> EGLRVVNLLQERNMLPST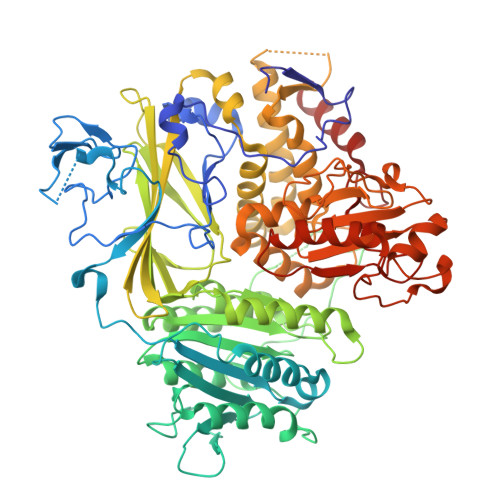PLKPPVPNLHEDIQKLNCNPELFRCTLTSIPQTQALLNKAKLPLGLLLHPFKDLVQLPVVTSSTIVRCRSCRTYINPFVSFLDQRRWKCNLCYRVNDVPEEFLYNPLTRVYGEPHRRPEVQNATIEFMAPSEYMLRPPQPPVYLFVFDVSHNAVETGYLNSVCQSLLDNLDLLPGNTRTKIGFITFDSTIHFYGLQESLSQPQMLIVSDIEDVFIPMPENLLVNLNESKELVQDLLKTLPQMFTKTLETQSALGPALQAAFKLMSPTGGRMSVFQTQLPTLGVGALKPREEPNHRSSAKDIHMTPSTDFYKKLALDCSGQQVAVDLFLLSGQYSDLASLGCISRYSAGSVYYYPSYHHQHNPVQVQKLQKELQRYLTRKIGFEAVMRIRCTKGLSIHTFHGNFFVRSTDLLSLPNVNPDAGYAVQMSVEESLTDTQLVSFQSALLYTSSKGERRIRVHTLCLPVVSTLNDVFLGADVQAISGLLANMAVDRSMTASLSDARDALVNAVIDSLSAYRSSVLSNQQPGLMVPFSLRLFPLFVLALLKQKSFQTGTNARLDERIFAMCQVKNQPLVYLMLTTHPSLYRVDNLSDEGALNISDRTIPQPPILQLSVEKLSRDGAFLMDAGSVLMLWVGKNCTQNFLSQVLGVQNYASIPQPMTDLPELDTPESARIIAFISWLREQRPFFPILYVIADESPMKANFLQNMIEDRTESALSYYEFLLHIQQQVNK> MQTGRTEDDLVPTAPSLGTKEGYLTKQGGLVK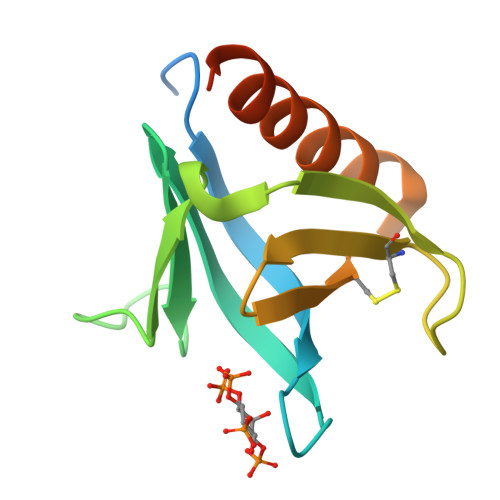TWKTRWFTLHRNELKYFKDQMSPEPIRILDLTECSAVQFDYSQERVNCFCLVFPFRTFYLCAKTGVEADEWIKILRWKLSQIRKQLNQGEGTIR> MRALLPYLALYKRHKWMLSLGIVLAIVTLLASIGLLTLSGWFLSASAVAGVAGLYSFNYMLPAAGVRGAAITRTAGRYFERLVSHDATFRVLQHLRIYTFSKLLPLSPAGLARYRQGELLNRVVADVDTLDHLYLRVISPLVGAFVVIMVVTIGLSFLDFTLAFTLGGIMLLTLFLMPPLFYRAGKSTGQNLTHLRGQYRQQLTAWLQGQAELTIFGASDRYRTQLENTEIQWLEAQRRQSELTALSQAIMLLIGALAVILMLWMASGGVGGNAQPGALIALFVFCALAAFEALAPVTGAFQHLGQVIASAVRISDLTDQKPEVTFPDTQTRVADRVSLTLRDVQFTYPEQSQQALKGISLQVNAGEHIAILGRTGCGKSTLLQQLTRAWDPQQGEILLNDSPIASLNEAALRQTISVVPQRVHLFSATLRDNLLLASPGSSDEALSEILRRVGLEKLLEDAGLNSWLGEGGRQLSGGELRRLAIARALLHDAPLVLLDEPTEGLDATTESQILELLAEMMREKTVLMVTHRLRGLSRFQQIIVMDNGQIIEQGTHAELLARQGRYYQFKQGL;> MNKSRQKELTRWLKQQSVISQRWLNISRLLGFVSGILIIAQAWFMARILQHMIMENIPREALLLPFTLLVLTFVLRAWVVWLRERVGYHAGQHIRFAIRRQVLDRL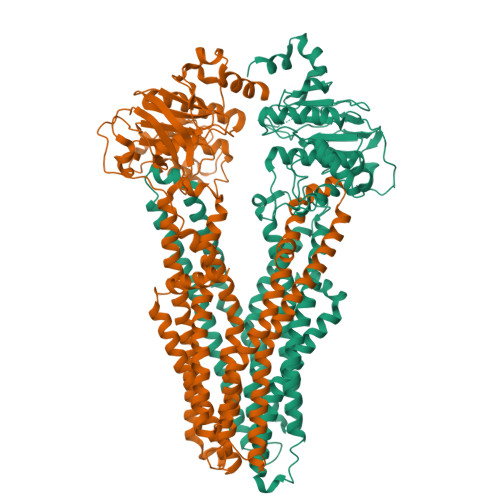QQAGPAWIQGKPAGSWATLVLEQIDDMHDYYARYLPQMALAVSVPLLIVVAIFPSNWAAALILLGTAPLIPLFMALVGMGAADANRRNFLALARLSGHFLDRLRGMETLRIFGRGEAEIESIRSASEDFRQRTMEVLRLAFLSSGILEFFTSLSIALVAVYFGFSYLGELDFGHYDTGVTLAAGFLALILAPEFFQPLRDLGTFYHAKAQAVGAADSLKTFMETPLAHPQRGEAELASTDPVTIEAEELFITSPEGKTLAGPLNFTLPAGQRAVLVGRSGSGKSSLLNALSGFLSYQGSLRINGIELRDLSPESWRKHLSWVGQNPQLPAATLRDNVLLARPDASEQELQAALDNAWVSEFLPLLPQGVDTPVGDQAARLSVGQAQRVAVARALLNPCSLLLLDEPAASLDAHSEQRVMEALNAASLRQTTLMVTHQLEDLADWDVIWVMQDGRIIEQGRYAELSVAGGPFATLLAHRQEEI> LGSPGIQGEVVDCHLSDMLQQLHSVNASKPSERGLVRQEEAEDPACIPIFWVSKWVDYSDKYGLGYQLCDNSVGVLFNDSTRLILYNDGDSLQYIERDGTESYLTVSSHPNS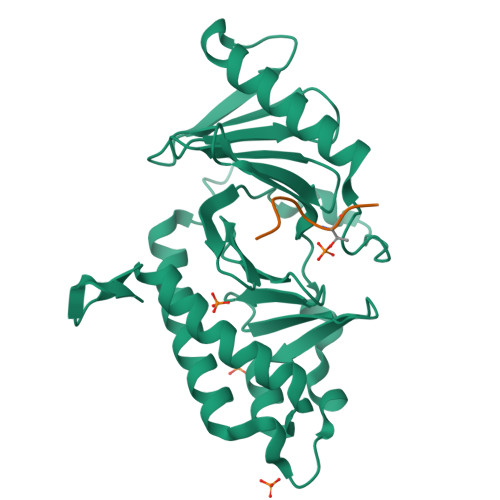LMKKITLLKYFRNYMSEHLLKAGANITPREGDELARLPYLRTWFRTRSAIILHLSNGSVQINFFQDHTKLILCPLMAAVTYIDEKRDFRTYRLSLLEEYGCCKELASRLRYARTMVDKLLSSRSASNRLKAS;> GPMTSTPK> ALLDETPLPPGSRLDVRAYTTVLHALSRAGRYERALELFAELRRQGVAPTVVTYNTLIDGLCKAGKLDEALKLFEEMVEKGIKPDVVTYNTLIDGLCKAGKL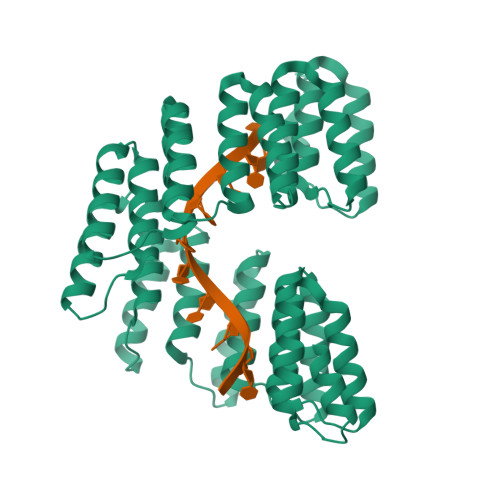DEALKLFEEMVEKGIKPDVVTYNTLIDGLCKAGKLDEALKLFEEMVEKGIKPDVVTYNTLIDGLCKAGKLDEALKLFEEMVEKGIKPDVVTYNTLIDGLCKAGKLDEALKLFEEMVEKGIKPSVVTYNTLIDGLCKAGKLDEALKLFEEMVEKGIKPSVVTYNTLIDGLCKAGKLDEALKLFEEMVEKGIKPDVVTYNTLIDGLCKAGKLDEALKLFEEMVEKGIKPDVVTYNTLIDGLCKAGKLDEALKLFEEMVEKGIKPDVVTYNTLIDGLCKAGKLDEALKLFEEMVEKGIKPDELTYRRVVESYCRAKRFEEARGFLSEVSETDLDFDKKALEAYIEDAQFGRLEHHHHHHHH>[4x]GPLGSPEFQKTKPFSVPNLPLNTLSNSRVPSLIRSMMVSRDHGQMVQFQNGRVTLDGQLQGTTPTSASQLCKIRGSVFHANGGNGYNLTELDGSPYHAFESPAPIGFPDLGECDWHMEASPTTQFDTGDVIKQINVKQEAAFAPHLGTIQADGLSDVSVNTNMIAKLGWVSPASDGHRGNVDPWVIPRYGSTLTEAAQLAPPIYPPGFGEAIVFFMSDFPIAHGANGLSVPCTIPQEFVTHFVNEQAPTRGEAALLHYLDPDTHRNLGEFKLYPEGFMTCVPNSSGTGPQTLPINGVFVFVSWVSRFYQLKPVGTAGPARSLGIRRS

NoV VP1 can be divided into two major domains: the N-terminal shell (S) domain and the C-terminal protruding (P) domain. The P domains form the outermost, dimeric protrusions of NoV virions, which plays critical roles in receptor recognition and host immune responses. HuNoVs recognize human histo-blood group antigens (HBGAs) as host receptors or attachment factors that play an important role in huNoV host susceptibility. In this study, we provided both phenotypic and structural evidence to show that huNoV DSV and VA115 recognize a group of glycans with terminal galactoses as ligands.

The crystal structure of native VA115 P protein was determined at 2.18 Å resolution, containing four VA115 P protein protomers or two homodimers in the crystallographic asymmetric unit. Most residues of VA115 P protein were modeled except residues S409–A415 (in B chain), due to uninterpretable local electron density maps caused by the local disorder of this highly flexible loop region. The two P proteins exhibited the typical huNoV P dimer arch-like structure with the P1 subdomains situated at the bottom and the P2 subdomain situated at the top. The major structural differences compared with other known P proteins are at the surface exposed loops, including the previously identified A-, B-, P-, T-, and U-loops in the P2 subdomain and the S-loop in the P1 subdomain. These variable loops confer DSV and VA115 unique surface topology from other huNoVs. We noted that the P-loop and T-loop on the surface of DSV/VA115 P protein exhibit a higher extension and the distance between the two loops becomes closer. Therefore, the glycan binding pocket becomes narrower but deeper, which hinders the binding to HBGAs. No complex was formed by soaking native VA115 P protein crystals with NA2 N-Glycan, probably due to crystal packing.> GSHMKNSVSVDLPGSMKVLVSKSSNADGKYDLIATVDALELSGTSDKNNGSGVLEGVKADASKVKLTISDDLGQT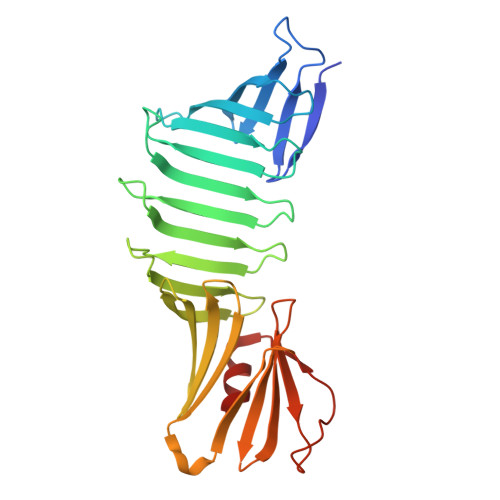TLEVFKSDGSTLVSKKVTSKDKSSTEEKFNEKGEVSEKIITRADGTRLEYTGIKSDGSGKAKEVLKGYVLEGTLTAEKTTLVVKEGTVTLSKNISKSGAVSVELNDTDSSTKKTAAWNSGTSTLTITVNSKKTKDLVFTSSNTITVQQYDSNGTSLEGSAVEITKLDEIKNALK>MAEFRIAQDVVARENDRRASALKEDYEALGANLARRGVDIEAVTAKVEKFFVAVPSWGVGTGGTRFARFPGTGEPRGIFDKLDDCAVIQQLTRATPNVSLHIPWDKADPKELKARGDALGLGFDAMNSNTFSDAPGQAHSYKYGSLSHTNAATRAQAVEHNLECIEIGKAIGSKALTVWIGDGSNFPGQSNFTRAFERYLSAMAEIYKGLPDDWKLFSEHKMYEPAFYSTVVQDWGTNYLIAQTLGPKAQCLVDLGHHAPNTNIEMIVARLIQFGKLGGFHFNDSKYGDDDLDAGAIEPYRLFLVFNELVDAEARGVKGFHPAHMIDQKHNVTDPIESLINSANEIRRAYAQALLVDRAALSGYQED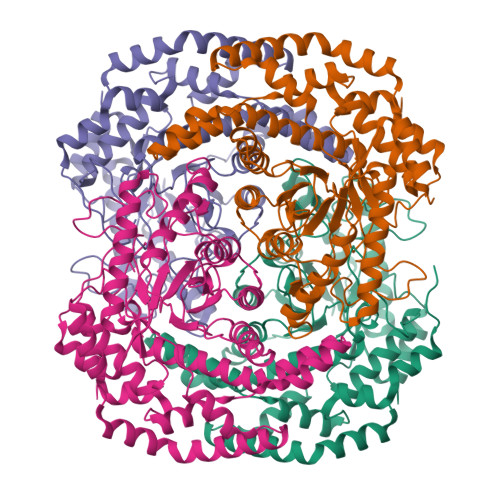NDALMATETLKRAYRTDVEPILAEARRRTGGAVDPVATYRASGYRARVAAERPASVAGGGGIIGSHHHHHH[4x]>[2x]MSSLLNSLLPEYFKPKTNLNINSSRVQYGFNARIDMQYEDDSGTRKGSRPNAFMSNTVAFIGNYEGIIVDDIPILDGLRADIFDTHGDLDMGLVEDALSKSTMIRRNVPTYTAYASELLYKRNLTSLFYNMLRLYYIKKWGSIKYEKDAIFYDNGHACLLNRQLFPKSRDASLESSLSLPEAEIAMLDPGLEFPEEDVPAILWHGRVSSRATCILGQACSEFAPLAPFSIAHYSPQLTRKLFVNAPAGIEPSSGRYTHEDVKDAITILVSANQAYTDFEAAYLMLAQTLVSPVPRTAEASAWFINAGMVNMPTLSCANGYYPALTNVNPYHRLDTWKDTLNHWVAYPDMLFYHSVAMIESCYVELGNVARVSDSDAINKYTFTELSVQGRPVMNRGIIVDLTLVAMRTGREISLPYPVSCGLTRTDALLQGTEIHVPVVVKDIDMPQYYNAIDKDVIEGQETVIKVKQLPPAMYPIYTYGINTTEFYSDHFEDQVQVEMAPIDNGKAVFNDARKFSKFMSIMRMMGNDVTATDLVTGRKVSNWADNSSGRFLYTDVKYEGQTAFLVDMDTVKARDHCWVSIVDPNGTMNLSYKMTNFRAAMFSRNKPLYMTGGSVRTIATGNYRDAAERLRAMDETLRLKPFKITEKLDFRVAAYAIPSLSGSNMPSLHHQEQLQISEVDAEPINPIGEDELPPDIE

L-BC virus persists in the budding yeast Saccharomyces cerevisiae, whereas other viruses from the family Totiviridae infect a diverse group of organisms including protists, fungi, arthropods, and vertebrates. Totiviridae is a family of viruses with monopartite double-stranded RNA (dsRNA) genomes, which contain two open reading frames encoding the capsid protein and the RNA-dependent RNA-polymerase (RdRp). The capsid of L-BC is organized with icosahedral symmetry with two subunits of capsid protein, named A and B, forming the icosahedral asymmetric unit. Decamers of capsid proteins are stabilized by domain swapping of the C-termini of subunits located around icosahedral fivefold axes.

Two-dimensional classification of particle images from a purified L-BC virus sample identified 87% empty particles, 9% open particles, and 4% genome-containing virions. The structure of the empty particle was determined to a resolution of 2.9 Å, whereas those of open particles and virions to 10 and 3.7 Å, respectively. dProtein geometry was refined against the reconstruction of the empty particle. However, the purified L-BC sample contained 87% empty particles and only 4% virions. This indicates that during the sample preparation, the fraction of empty particles was enriched or the genome release was induced. The observed particle damage could have been induced by the freeze-thaw cycle required for sample shipping or the low ionic strength of the buffer (20 mM Tris-HCl pH 7.5, 50 mM KCl, 10 mM MgCl2) used during particle vitrification. The alpha-helical cores of L-BC A and B subunits have nearly identical structures, which can be superimposed with RMSD of 0.6 Å. The strand βU of the A1 subunit is inserted between the strands βJ and βK of the A2 subunit related by 72° counterclockwise rotation when looking from the inside of the particle. These strand insertions between adjacent A subunits propagate around the fivefold symmetry axis and may stabilize the decamer structure. Salt bridges at two positions stabilize the domain swap between A subunits.(5R)-5-methyl-5-[[(1R,2R,5R)-2-methyl-5-(3-oxidanylideneprop-1-en-2-yl)cyclopentyl]methyl]-2-propan-2-yl-cyclopenta-1,3-diene-1-carboxylic 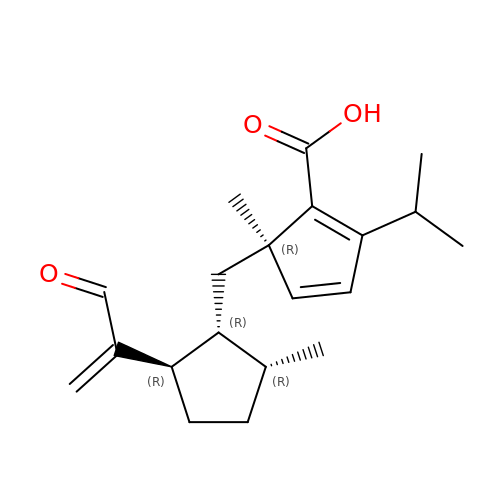acid | C20 H28 O3 | CSCGDRYDSLORNR-UDUZWTERSA-N> HHHHHHMQPGGDMSALLAQAQQMQQKLLEAQQQLANSEVHGQAGGGLVKVVVKGSGEVIGVTIDPKVVDPDDIETLQDLIVGAMRDASQQVTKMAQ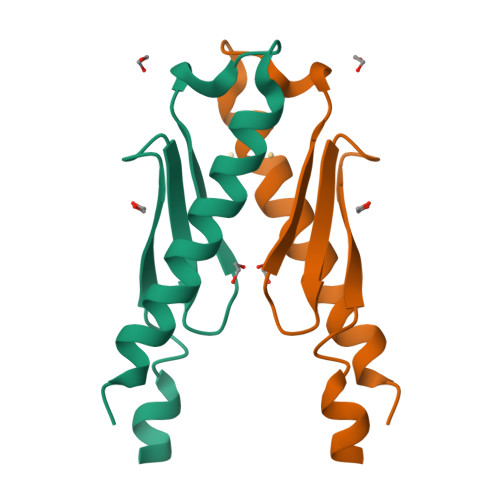ERLGALAGAMRPPAPPAAPPGAPGMPGMPGMPGAPGAPPVPGI> GESEDDKAFEENRRLRN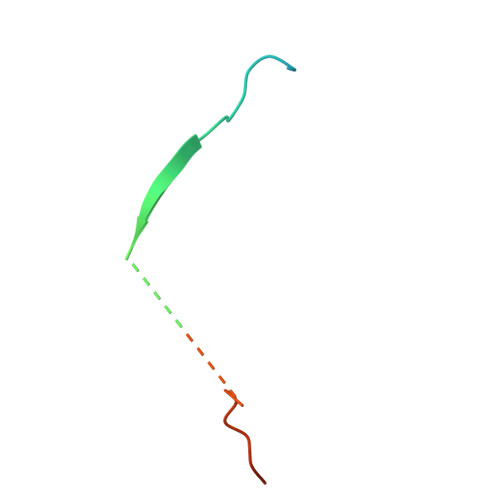LGSVEYIRIMSSEKSNANSRHTSKYYSGRKNFKKFQKKASQK(3R)-3-[(R)-[(2R,6S)-6-methyloxan-2-yl]-oxidanyl-methyl]-6,8-bis(oxidanyl)-3,4-dihydroisochromen-1-one 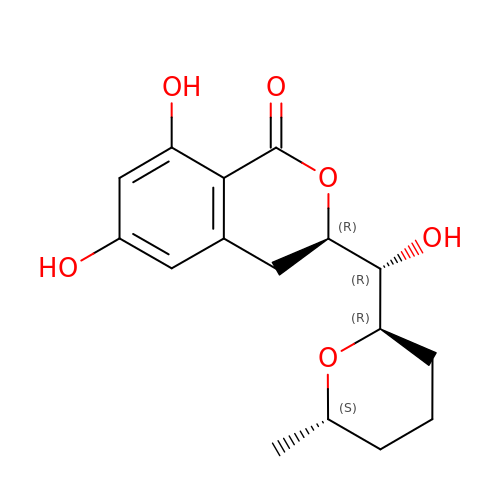| C16 H20 O6 | YVPGTQQTPNCAJJ-VFJFRJDUSA-N>[8x]CG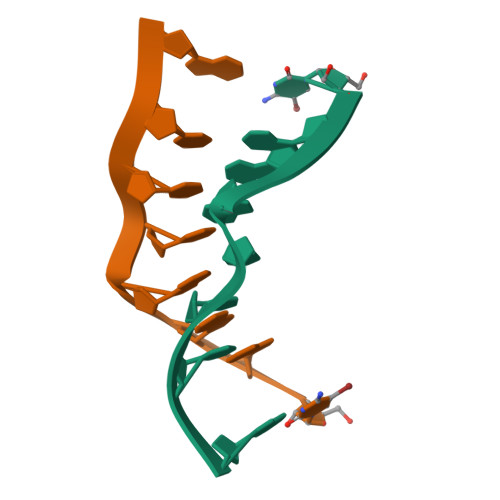AAXUCG>[2x]MRGSHHHHHHGSASFLKKTMPFK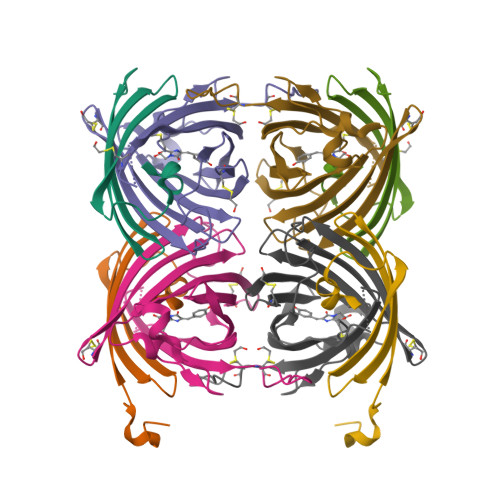TTIEGTVNGHYFKCTGKGEGNPFEGTQEMKIEVIEGGPLPFAFHILSTSCX;>[2x]MYGSKTFIKYVSGIPDYFKQSFPEGFTWERTTTYEDGGFLTAHQDTSLDGDCLVYKVKILGNNFPADGPVMQNKAGRWEPGTEIVYEVDGVLRGQSLMALKCPGGRHLTCHLHTTYRSKKPASALKMPGFHFEDHRIEIMEEVEKGKCYKQYEAAVGRYCDAAPSKLGHN> HHH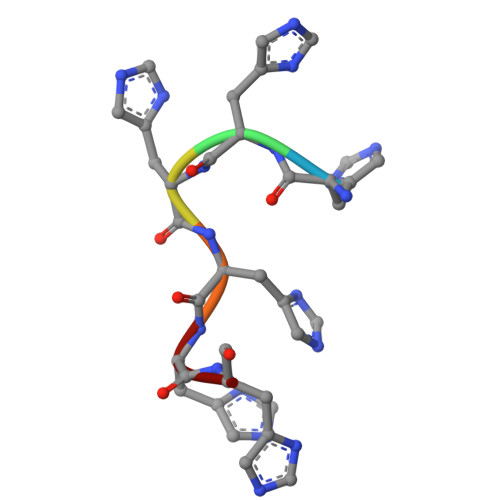HHH Chalcone isomerase–like (CHIL) protein is a noncatalytic protein that enhances flavonoid content in green plants by serving as a metabolite binder and a rectifier of chalcone synthase (CHS). Rectification of CHS catalysis occurs through direct protein–protein interactions between CHIL and CHS, which alter CHS kinetics and product profiles, favoring naringenin chalcone (NC) production. The chalcone isomerase–like (CHIL) protein family is noncatalytic, yet it shares a “CHI fold” with CHI. The protein X-ray crystal structures of PpCHIL-A and VvCHIL reveal CHI-type α/β folds with high structural homology to each other.

When the structures of VvCHIL and MtCHI-I bound with naringenin are aligned, a significant amount of the VvCHIL pocket is occluded. Most notably, tryptophan 221 (W221) and glutamine 141 (Q141) produce overlaps with naringenin. Nearby to the tryptophan in the structure of VvCHIL, a glutamine (Q141) also occupies the canonical binding site, yet this glutamine is not highly conserved across CHIL sequences. On the other hand, the presence of the tryptophan and glutamine side chains create a fundamentally different chemical topography for the VvCHIL-binding pocket, potentially changing the nature of ligand interactions. Supporting this idea, analysis of the VvCHIL-binding pocket reveals a pocket volume of 20.8 A3, whereas the volume of the PpCHIL-A–binding pocket is significantly larger, calculated to be 50.7 A3. The comparison of VvCHIL and PpCHIL-A protein crystal structures suggests that W221 may be responsible for the destabilizing effect to VvCHIL caused by naringenin binding. With the W221L substitution in place, VvCHIL does not undergo thermal destabilization in the presence of naringenin. Similarly, a variant of VvCHIL with the Q141A substitution does not undergo thermal destabilization in the presence of naringenin, suggesting W221 and Q141 together are required to facilitate destabilization. For VvCHIL, naringenin binding produces the opposite effect on the thermal shift relative to PpCHIL-A and MsCHI-II, resulting in reduced protein Tms at high naringenin concentrations. The VvCHIL peaks calculate to 26 kDa (major peak) and 68 kDa (minor peak), indicating that a minor amount of VvCHIL is stable as a multimer, perhaps as a trimer in this experiment.

> RGSHGGSMGTEMVMVDEIPFPPQITTAKPLCLLGYGITDIEIHFLQIKFTAIGVYLEPEIVGHLQPWKGKSGKELAENDDFFEALISAPGEKFLRIVVIKEIKGSQYGVQLESAVRDRLAADDKYEEEEEEALEKVVEFFQSKYFKKDSIITFHFPATSFTAEIVFATEGKEESKITVENANVVEMIKKWYLGGTRGVSPTTISALANTLATELSK> MRNQFDLELHELEQSFLGLGQLVLETASKALLALASKDKEMAELIINKDHAINQGQSAIELTCARLLALQQPQVSDLRFVISIMSSCSDLERMGDHMAGIAKAVLQLKENQLAPDEEQLHQMGKLSLSMLADLLVAFPLHQASKAISIAQKDEQIDQYYYALSKEIIGLMKDQETSIPNGTQYLYIIGH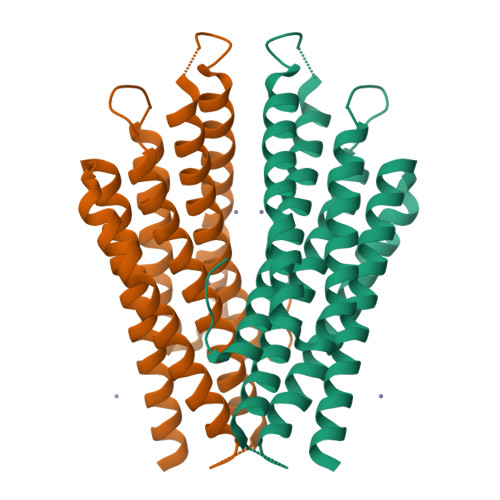LERFADYIANICERLVYLETGELVDLN>[2x]MERDGCAGGGSRGGEGGRAPREGPAGNGRDRGRSHAAEAPGDPQAAASLLAPMDVGEEPLEKAARARTAKDPNTYKVLSLVLSVCVLTTILGCIFGLKPSCAKEVKSCKGRCFERTFGNCRCDAACVELGNCCLDYQETCIEPEHIWTCNKFRCGEKRLTRSLCACSDDCKDKGDCCINYSSVCQGEKSWVEEPCESINEPQCPAGFETPPTLLFSLDGFRAEYLHTWGGLLPVISKLKKCGTYTKNMRPVYPTKTFPNHYSIVTGLYPESHGIIDNKMYDPKMNASFSLKSKEKFNPEWYKGEPIWVTAKYQGLKSGTFFWPGSDVEINGIFPDIYKMYNGSVPFEERILAVLQWLQLPKDERPHFYTLYLEEPDSSGHSYGPVSSEVIKALQRVDGMVGMLMDGLKELNLHRCLNLILISDHGMEQGSCKKYIYLNKYLGDVKNIKVIYGPAARLRPSDVPDKYYSFNYEGIARNLSCREPNQHFKPYLKHFLPKRLHFAKSDRIEPLTFYLDPQWQLALNPSERKYCGSGFHGSDNVFSNMQALFVGYGPGFKHGIEADTFENIEVYNLMCDLLNLTPAPNNGTHGSLNHLLKNPVYTPKHPKEVHPLVQCPFTRNPRDNLGCSCNPSILPIEDFQTQFNLTVAEEKIIKHETLPYGRPRVLQKENTICLLSQHQFMSGYSQDILMPLWTSYTVDRNDSFSTEDFSNCLYQDFRIPLSPVHKCSFYKNNTKVSYGFLSPPQLNKNSSGIYSEALLTTNIVPMYQSFQVIWRYFHDTLLRKYAEERNGVNVVSGPVFDFDYDGRCDSLENLRQKRRVIRNQEILIPTHFFIVLTSCKDTSQTPLHCENLDTLAFILPHRTDNSESCVHGKHDSSWVEELLMLHRARITDVEHITGLSFYQQRKEPVSDILKLKTHLPTFSQED

Ectonucleotide pyrophosphatase/phosphodiesterase 1 (ENPP1) is an emerging therapeutic target in human cancers owing to its role in degrading cyclic GMP-AMP (cGAMP), an agonist of the stimulator of interferon genes (STING). Ectonucleotide pyrophosphatase/phosphodiesterase 1 (ENPP1), also known as PC-1, is found as a secreted protein in the extracellular matrix and as a membrane-bound protein intracellularly and on the cell surface. ENPP1 has a role in purin­ergic signalling through the hydrolysis of nucleotide triphosphates (NTPs) and cyclic nucleotides (cNMPs) to their corresponding nucleotide monophosphates (NMPs). Apart from viral poxins, ENPP1 is the only known hydrolase of cyclic GMP-AMP (cGAMP), which is a second messenger generated by cyclic GMP-AMP synthase (cGAS) as an innate immune-system response to double-stranded DNA in the cytosol.

ADU-S100 is a STING agonist that is currently in clinical trials, while QPS2 and Ex54 are published ENPP1 inhibitors. The fused rings of QPS2 and Ex54 occupy the same region as the adenine of AMP but extend further into the pocket, displacing the waters that hydrogen-bond to N6 of AMP. The quin(az)oline projects deeper into the pocket than the adenine ring, making additional interactions with Phe321, Pro323, Asp326 and Tyr371. In the AMP-bound structure, two water molecules are hydrogen-bonded to the N6 position. These are displaced in the QPS2-bound and Ex54-bound structures, and a hydrogen bond between the 7-methoxy group and Trp322 is introduced (3.0–3.2 Å). The methoxy moiety also appears in close contact with the carbonyl of Trp322 (2.4–2.8 Å), which may offset the affinity gains from the introduced hydrogen bond. Ex54 and QPS2 extend out of the adenine pocket via benzene and piperidine rings, respectively, which occupy a similar space to that of the ribose ring of AMP. The sulfamide groups of QPS2/Ex54 do not project towards the zinc site (as per the phosphate of AMP), but instead form hydrogen bonds to Glu373, Asp376 and Ser377. The sulfamide of Ex54 is flipped in the B protomer, projecting towards the bound phosphate, and therefore does not make the above inter­actions. The sulfamide moieties of these inhibitors do not seem to make strong interactions in the catalytic site, unlike the phosphate of AMP.> HHHHHHEVLLRSTETGQFLRINPDGTVDGTRDRSDPGIQFQISPEGNGEVLLRSTE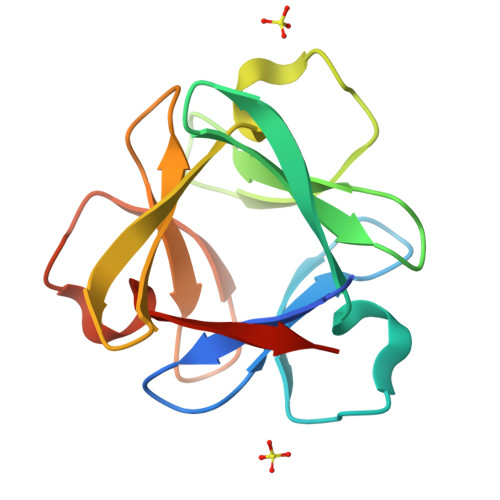TGQFLRINPDGTVDGTRDRSDPGIQFQISPEGNGEVLLRSTETGQFLRINPDGTVDGTRDRSDPGIQFQISPEGNG> NNDDPVENFVESTLKEVLVVPDTKPSGPQHTTKPSILGAMEIGASSNATPESTIETRYVYNTNTNAEADVEMFLGRSALWGKVTLTRQYAKWEINFQEQAHIRKKFEFFTYLRFDM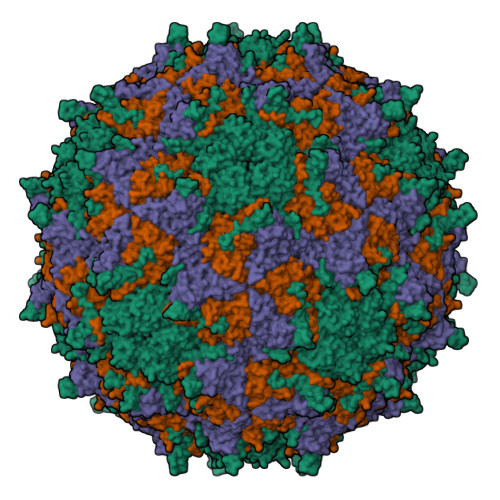EVTIVTNNKGLMQIMFVPPGIDHPETHDDRKWDSASNPSVFFQPKSGFPRFTIPFTGLASAYYMFYDGYDKPKGSDNNEYGIAPTNDMGLLCFRTLDNSGGNDVKIYVKPKHITAWVPRPPRATQYTHKYSTNYHYKPNSSGPDEHVLKDRHFIKTRPLISSA;> GLPTRLPSGSQQFMTTEDEQSPNILPGFHPSKKIHIPGMITNVMHMARVDSFIPINNIQGEVGKVSMYYITVTKKTVTERILVLPLEMSNTLFATTLLGEVLNYYANWSGSITITFMCVCDAFSTGKFLVAYTPPGGKLPEDRKQAMLGVHIIWDLGLQSSCTIVVPWISSGFYRRTKADSFTHGGYVSLWYQTAFVPPVSGGTGSILATCSACPDMSVRMLRDSPMMEQKNELQ;> GAQVSRQNNGTHENGVTASNGSVIKYFNINYYKDSASSGLSRQDFSQDPSKFTQPLVDTLTNPALMSPSVEACGYSDRLKQITIGNSTITTQDSLHTVLAYGEWPTYLSDIDATSVDKPTHPETSADRFYTLDSVEWQVGSHGWWWKLPDALKDMGVFGQNMYYHSMGRSGFIIHTQCNATKFHSGALIVAVIPEHQLAYVGGVKVNVGYDHTHPGQSGHQIRGPSQSNDRSGGKPDEDPLFNCNGTLLGNITIFPHQIINLRTNNSSTIVVPYINCVPMDNMLKHNNLSLVIIPLVPLRPGSSGINSVPITVTIAPYKSEFSGAMEAQRQ>[2x]ADGKILHNQNV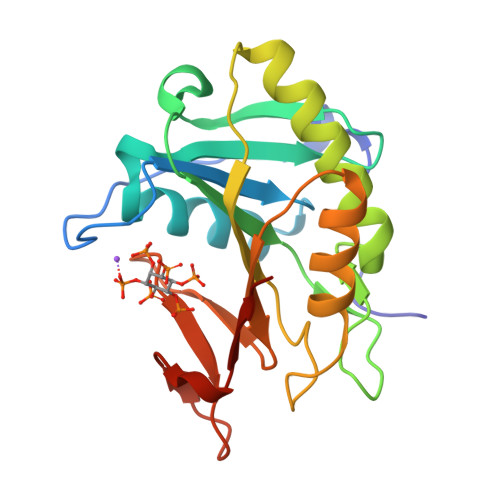NSWGPITVTPTTDGGETRFDGQIIVQMENDPVVAKAAANLAGKHAESSVVVQLDSDGNYRVVYGDPSKLDGKLRWQLVGHGRDHSETNNTRLSGYSADELAVKLAKFQQSFNQAENINNKPDHISIVGCSLVSDDKQKGFGHQFINAMDANGLRVDVSVRSSELAVDEAGRKHTKDANGDWVQKAENNKVSLSWDAQG>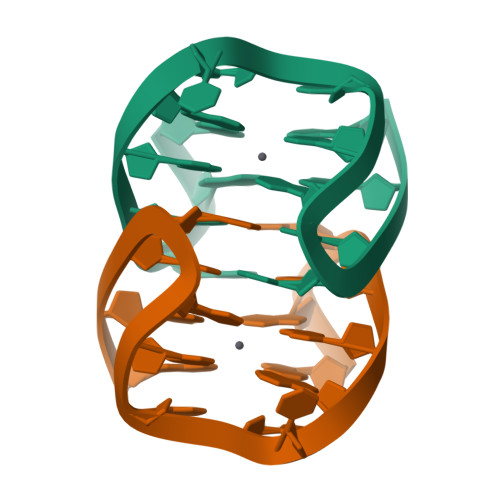GGTTGGTCTGGTTGG[5x]> MERTELLKPRTLADLIRILHELFAGDEVNVEEVQAVLEAYESNPAEWALYAKFDQYRYTRNLVDQG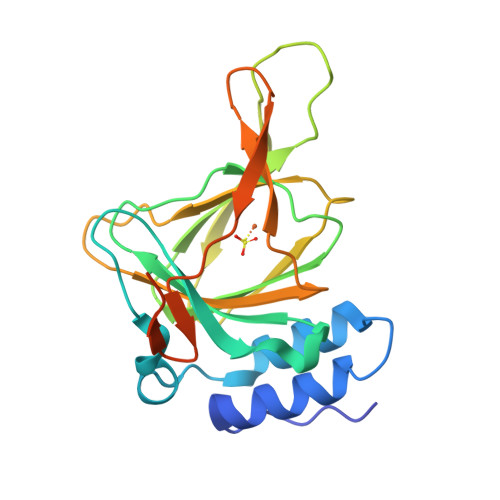NGKFNLMILCWGEGHGSSIHDHTDSHCFLKLLQGNLKETLFDWPDKKSNEMIKKSERTLRENQCAYINDSIGLHRVENVSHTEPAVSLHLHSPPFDTCHAFDQRTGHKNKVTMTFHSKFGIRTPFTTSGSLENNSAWSHPQFEK N-(4-bromo-3-methylbenzoyl)-4-[difluoro(phosphono)methyl]-L-phenylalanyl-N~5~-(3-iodobenzoyl)-L-ornithyl-3-{[(4-hydroxy-3-methoxyphenyl)acetyl]amino}-D-alaninamide 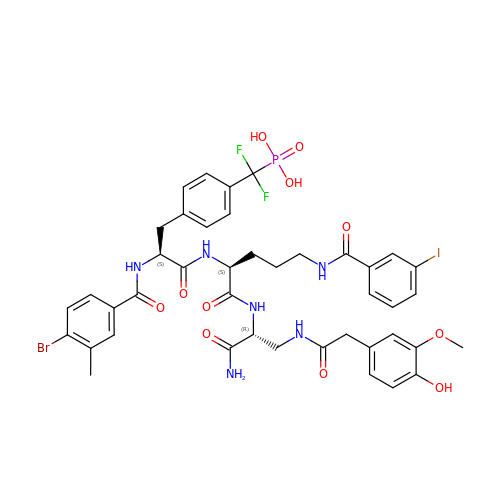| C42 H45 Br F2 I N6 O11 P | UUBNUVGMYMXEBE-XFCANUNOSA-N> MLRSSNDVTQQGSRPKTKLGGSSMGIIRTCRLGPDQVKSMRAALDLFGREFGDVATYSQHQPDSDYLGNLLRSKTFIALAAFDQEAVVGALAAYVLPKFEQPRSEIYIYDLAVSGEHRRQGIATALINLLKHEANALGAYVIYVQADY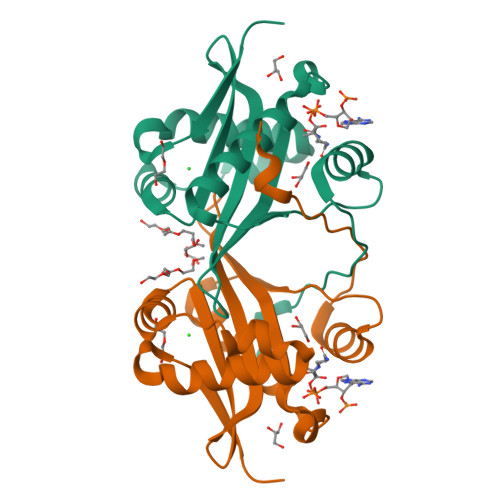GDDPAVALYTKLGIREEVMHFDIDPSTAT1-[6-(furan-2-yl)pyridin-3-yl]methanamine | C10 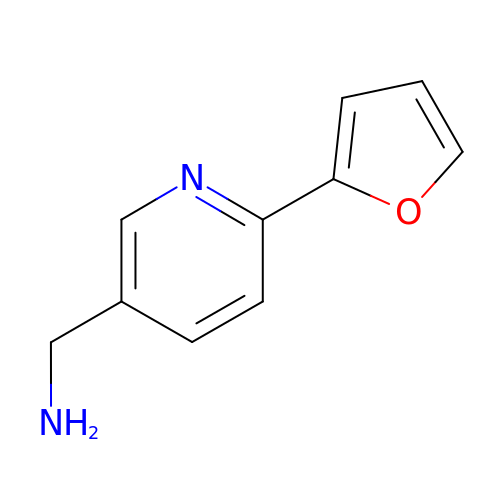H10 N2 O | WEPDEUMTQHBFOQ-UHFFFAOYSA-N(2E)-3-(3,4-DIHYDROXYPHENYL)-N-[2-(4-HYDROXYPHENYL)ETHYL]ACRYLAMIDE | C17 H17 N O4 | 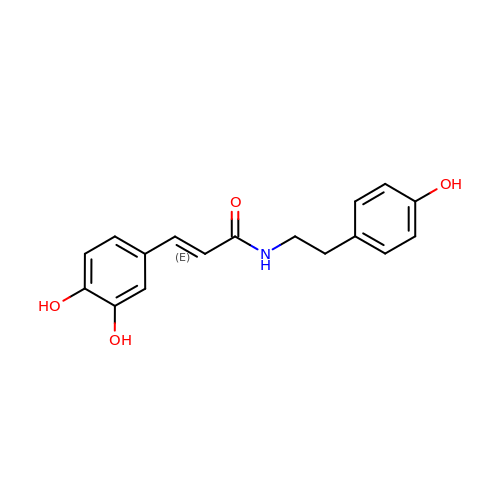VSHUQLRHTJOKTA-XBXARRHUSA-N(Z)-[(3R,4R,5R,6R)-3-acetamido-6-(hydroxymethyl)-4,5-bis(oxidanyl)oxan-2-ylidene]amino] N-phenylcarbamate | C15 H19 N3 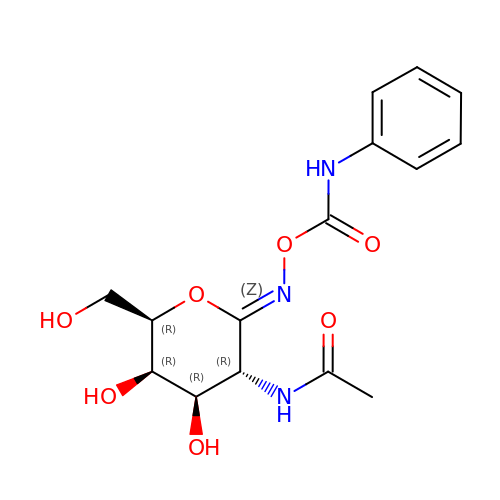O7 | PBLNJFVQMUMOJY-UYZOWNTJSA-N>[4x]MGSSHHH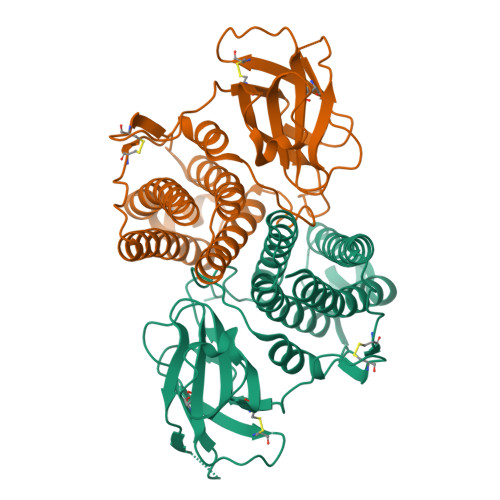HHHENLQFQGGGNRGMSRNQDAYAEKMDMTLDALNFLLGVEHLASAFYVQAVNNFTADDFKAAGLAQRDYDQFVGVRNNEVDHRDTLISVIKSLGGKPNPPCKYTFPVTDVASVLKVSRTLENADKPAYLGALRDIKSVELRTSVQGALSGDSAHAAFFAYLTGKAPAPGPVDGPLTQRHIATLAQDFIVSCPYPAPKPFPKLTLSPQSGPVGTVVATTCAQDVDTNGVMCAIISGNQGTLMQRPGQAKDGSGAATCTIPPGVKGILFIAWVRGRDVLNVGVDDSSTVCGPNYFLLSALGDAVPGV The human assembly factor Coa6 participates in the biogenesis of the CuA site in complex IV (cytochrome c oxidase, COX). Coa6 is a soluble IMS protein with a CX9C–CX10C sequence motif, which binds Cu(I) with a KD(CuI) of ∼10−17 M. Coa6 deletion in both yeast and human cells results in diminished COX assembly and activity; however, this defect can be partially rescued by exogenous copper supplementation and in yeast by treatment with elesclomol (via a proposed elesclomol–copper complex). Here, we present the crystal structures of human Coa6 and the pathogenic W59CCoa6-mutant protein. These structures show that Coa6 has a 3-helical bundle structure, with the first 2 helices tethered by disulfide bonds, one of which likely provides the copper-binding site. Patients with mutations in Coa6 suffer from mitochondrial disease due to complex IV deficiency.

Finally, we determined and refined the crystal structure of the pathogenic mutant protein W59CCoa6 to 2.2 Å resolution by X-ray crystallography. The structure of W59CCoa6 shows four molecules (A, B, C, and D) per asymmetric unit. The noncovalent dimer observed in the WTCoa6 structure is maintained for W59CCoa6 (between molecules A [cyan] and B [gray]) through contacts along Helix α3 from each monomer. In addition, each of these molecules form a covalent dimer with another molecule of W59CCoa6 through a disulfide bond between the introduced residue Cys59 on each chain (covalent dimers between molecules A/D, [cyan and salmon] and B/C [gray and gold], Fig 4B). In this way, the asymmetric unit is composed of a dimer of dimers (a noncovalent dimer of disulfide bridged dimers). The superposition of the WTCoa6 structure with the noncovalent A/B dimer of W59CCoa6 yields a r.m.s.d. value of 1.2 Å for 113 common Cα atoms. These minor structural differences originate from a slightly different association between the monomers in the dimers, rather than specific structural rearrangements. Importantly, in the WTCoa6 and W59CCoa6 structures, the positions of the proposed Cys58–Cys90 Cu(I)-binding sites are identical. Under reducing conditions, the elution profile for the W59CCoa6 protein was identical to that of WTCoa6, corresponding to a dimeric protein. These observations agree with the crystal structure described here, which shows that W59CCoa6 oligomerization is mediated by the presence of intermolecular disulfide bonds that bridge noncovalent W59CCoa6 dimers. Oligomerization of the protein, through the creation of intermolecular disulfide bonds may inhibit or eliminate targeted protein–protein interactions between Coa6 and proteins such as Sco1, Sco2, and COX2, which are critical for its function.

>[4x]APSMKERQVCCGARDEYWKCLDENLEDASQCKKLRSSFESSCPQQWIKYFDKRRDYLKFKEKFEA> SRSKKKT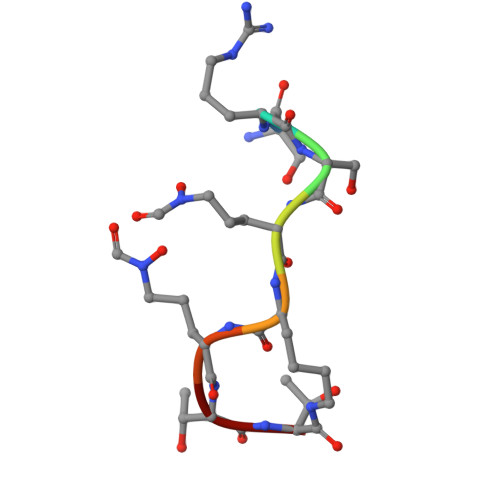T2-chloro-4-{[2-(4-methylpiperazin-1-yl)-3,4-dioxocyclobut-1-en-1-yl]amino}phenyl 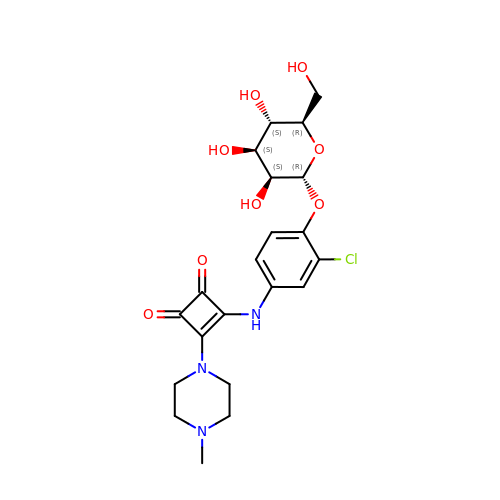alpha-D-mannopyranoside | C21 H26 Cl N3 O8 | OVFSRWMGARZIAS-YVNBQAQUSA-N>GPAMAKVETGTDVTSKVTVEIGSIEGHNNTNKVEPHAGQRAVLKYKLKFENGLHQGDYFDFTLSNNVNTHGVSTARKVPEIKNGSVVMATGEVLEGGKIRYTFTNDIEDKVDVTAELEINLFIDPKTVQTNGNQTITSTLNEEQTSKELDVKYKDGIGNYYANLNGSIETFNKANNRFSHVAFIKPNNGKTTSVTVTGTLMKGSNQNGNQPKVRIFEYLGNNEDIAKSVYANTTDTSKFKEVTSNMSGNLNLQNNGSYSLNIENLDKTYVVHYDGEYLNGTDEVDFRTQMVGHPEQLYKYYYDRGYTLTWDNGLVLYSNKA[2x];>GEGQQHHLGGAKQAGDV[2x]

The adjacent fibrinogen (Fg)- and fibronectin (Fn)-binding sites on Fn-binding protein A (FnBPA), a cell surface protein from Staphylococcus aureus, are implicated in the initiation and persistence of infection. The N-terminal region of FnBPA contains three subdomains N1–N3; N2N3 binds fibrinogen (Fg) and elastin. Here, we solved the structure of the N2N3 domains containing the Fg-binding site of FnBPA in the apo form and in complex with a Fg peptide. The Fg binding mechanism is similar to that of homologous bacterial proteins but without the requirement for “latch” strand residues.

The rFnBPA(189–505)·FgγC complex was solved using x-ray crystallography. The FgγC peptide binding site is located in a cleft between N2 and N3. FgγC forms an additional β-strand parallel to the G′ strand in N3 in a β-zipper interaction. The r.m.s.d between the structures of free and FgγC-bound rFnBPA(189–505) is 0.81 Å, confirming that binding of FgγC does not induce large conformational changes in the individual N2 and N3 domains or in their relative orientation. The translocation of the N3 G′ strand is the only significant change. In the FgγC-bound form, the G′ strand “wraps” around the C-terminal residues Gln-13, Ala-14, and Gly-15 of the peptide and interacts with the N2 domain. Tyr-501 and Asn-503, which protrude away from the unbound rFnBPA(189–505) structure, form hydrogen bonds with Gly-222 and Asn-304, respectively, in FgγC-bound rFnBPA(189–505). The combined buried surface area within the rFnBPA(189–505)·FgγC A·C chain interface is 1880 Å2. In contrast to the apo-protein structure, no electron density was detected within the N3 loop (residues 479–489) that connects the F′ and G′ strands. Clearly, the latch β-strand residues are absent in the FnBPA(189–505)·FgγC structure.3-[4-AMINO-1-(1-METHYLETHYL)-1H-PYRAZOLO[3,4-D]PYRIMIDIN-3-YL]PHENOL 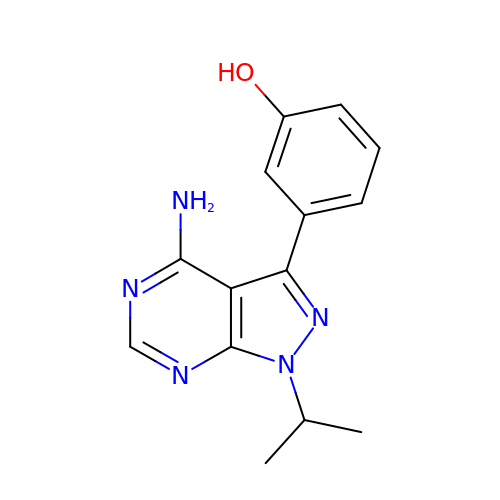| C14 H15 N5 O | MWYBBCLGEHZSCP-UHFFFAOYSA-N>HHHHHHMASSAQDGNNPLFSPYKMGKFNLSHRVVLAPMTRCRALNNIPQAALGEYYEQRATAGGFLITEGTMISPTSAGFPHVPGIFTKEQVREWKKIVDVVHAKGAVIFCQLWHVGRASHEVYQPAGAAPISSTEKPISNRWRILMPDGTHGIYPKPRAIGTYEISQVVEDYRRSALNAIEAGFDGIEIHGAHGYLIDQFLKDGINDRTDEYGGSLANRCKFITQVVQAVVSAIGADRVGVRVSPAIDHLDAMDSNPLSLGLAVVERLNKIQLHSGSKLAYLHVTQPRYVAYGQTEAGRLGSEEEEARLMRTLRNAYQGTFICSGGYTRELGIEAVAQGDADLVSYGRLFISNPDLVMRIKLNAPLNKPNRKTFYTQDPVVGYTDYPFLQGNGSNGPLSRL[2x]

Jasmonates are phytohormones that are pivotal in mediating plant responses to various biotic and abiotic stresses and regulating plant growth. The first crystal structure of OPR3 from tomato (SlOPR3) showed that the enzyme crystallized as a self-inhibitory dimer in which the L6 loop, a critical loop involved in substrate recognition and coenzyme binding, from each protomer intrudes into the active site cavity of the other protomer. Based on these observations, it was postulated that the formation of the self-inhibitory homodimer represents a mechanism for regulating OPR3 activity and, thereby, jasmonic acid biosynthesis.

Variant Y364P was produced to test whether residue Y364 is required for homodimerization, as proposed previously. Even variant Y364P, lacking the putative phosphorylation site, was crystallized as a self-inhibitory homodimer, indicating that Y364 is not required for dimerization. Despite missing a tyrosine residue at position 364 and a sulfate ion, SlOPR3 Y364P can still form the same homodimer, clearly positing against the proposed regulation of OPR3 activity by phosphorylation in vivo. The slight difference between the dimers arises from the protomers being differently positioned to each other. Thus, it seems unlikely that reverse phosphorylation of Y364 serves as a regulation mechanism in vivo.So far, there is only one described microbial system able to degrade molinate to innocuous compounds: a five strong bacteria consortium from which Gulosibacter molinativorax ON4T is responsible for the initial breakdown of the herbicide by cleaving its thioesther bond, releasing ethanethiol and azepane-1-carboxilate (ACA). This reaction is catalyzed by molinate hydrolase (MolA). Following successful identification and cloning of its encoding gene, recombinant molinate hydrolase was found to be cobalt-dependent, with zinc and manganese also able to confer activity to the enzyme. The structure of molinate hydrolase consists of a homotetramer composed of two symmetry-related dimers with a 67° tilt angle between them.

Good diffracting crystals of recombinant molinate hydrolase were obtained in two distinct crystal systems, orthorhombic and monoclinic, with 4 and 8 monomers in the asymmetric unit, respectively. Later on we solved a crystal structure partially loaded with one of the potential catalytic metal ions, Zn2+, by co-crystallizing the recombinant enzyme with ZnCl2. The position of the metal ions was determined from single wavelength anomalous diffraction data collection at the Zn absorption K-edge. The anomalous signal was modest but the top positive peaks in the anomalous difference Fourier map were located in equivalent positions in each monomer and were consistent with metal coordination geometry and with the position of the metal ions in structure-related amidohydrolases. The Zn ions occupation was set to 0.4 and the overall structure was similar to the one of the metal–free enzyme (root-mean-squared-distance r.m.s.d. of the superimposed structures is 0.22 Å). The active site structure was also not perturbed by the depletion of the catalytic metal ion. The catalytic metal is coordinated by His282 and His302 (residues are numbered according to the recombinant protein sequence, including a 32 amino acid purification tag), which are hydrogen-bonded to the main chain carbonyl groups of Asp245 and Thr283, respectively, as well as three ordered water molecules. The water molecules are in turn hydrogen-bound to Lys240, His246 and Asp373.

>[8x]MASWSHPQFEKIEGRRDRGPEFELGTENLFFEGETIAIVGGTLIDGNGGVPVPETTVFIEDGRITKVGSTDQIEVHPNIRQIDAQGKWILPGLVNGNVHLLDGIMMMGRGGIEYLARFEGNYYKVIEEAAQIALRGGVTTVFDTWNALEPVTIARDRIASGAAEGARIFFAGTLIGMGGPFTGDFMRPSMQARTVMSRTFADRMDAMFEVGMGRHLSTLPPAEVRPLIREYLERGVDFCKIAVTDHLVGLLGFRAPYFTFSERVLDVLVDEVRRAGVPLLTHTTSLEGLNTAIERDADLMIHATMTGQAPIPEETIEKLLEKQLWSEVQPTTIAQQAWMDSVDHPFADFSGRVHHENDVRMIKAGVPLVLGTDAGCTDPDILEDMSQGELHERPWTLGEDHFVWMQAMVEKGMDPMAAILAGTANPAKAYRKFDELGSIDVGKLGDVVVLDQDPLADITNMRTLSHVVKEGREIDFHGLPLSPLVTAYPRTANVLD> MMRFAIAAALGALLAVAAAPAAVAAARRPPWDIARFRPALRVAKLQAPDSVQRKDVRSFPNFQADHFYSENRDMVFVMGGDSQRSELRFLDEWSVRTSSTRRMVGVLTLPTPLRGMKHFTWMQVAGGSKGKKPLL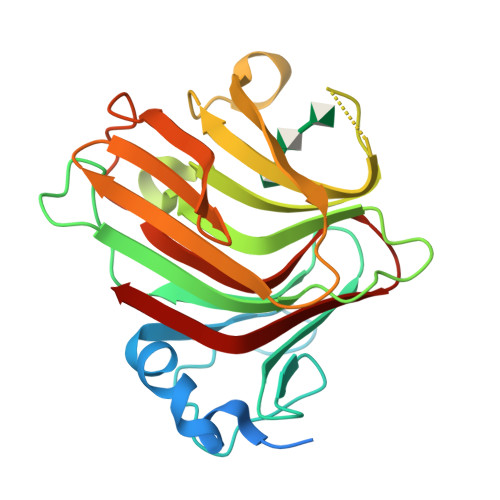RLSWHDKREQGGKDLRNTMLATVRLNNKSGDAGRFKKIVLGTRPSGRFVADVRVERSRLTVRLNGRKLVDEDVGYWTYSTNYFKAGVYVQEGSPDARVVFHGLTVS> GSKHVKKVYSCDLTTLVKAHTTKRPMVVD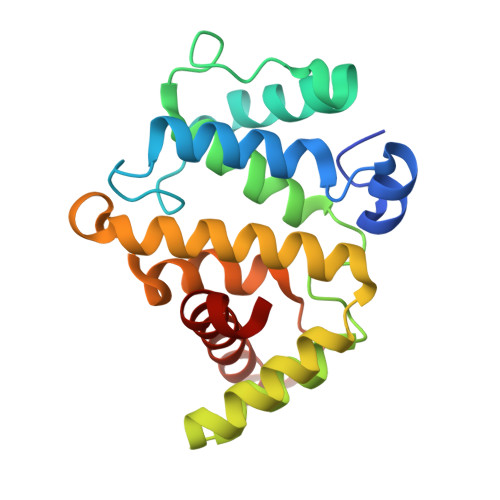MCIREIESRGLNSEGLYRVSGFSDLIEDVKMAFDRDGEKADISVNMYEDINIITGALKLYFRDLPIPLITYDAYPKFIESAKIMDPDEQLETLHEALKLLPPAHCETLRYLMAHLKRVTLHEKENLMNAENLGIVFGPTLMRSPELDAMAALNDIRYQRLVVELLIKNEDILF> ATVAAYNLTWKSTNFKTILEWEPKPVNQVYTVQISTKSGDWKSKCFYTTDTECDLTDEIVKDVKQTYLARVFSYPAGNVESTGSAGEPLYENSPEF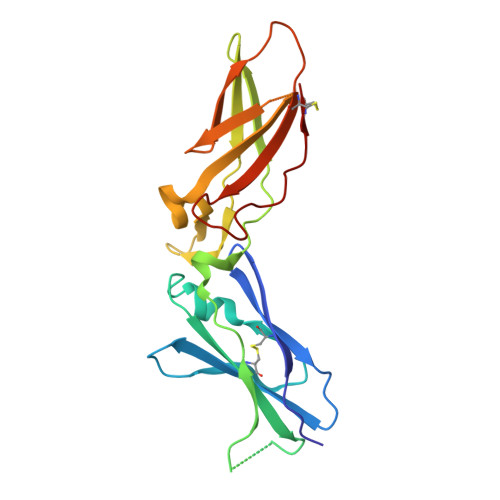TPYLETNLGQPTIQSFEQVGTKVNVTVEDERTLVRRNNTFLSLRDVFGKDLIYTLYYWKSSSSGKKTAKTNTNEFLIDVDKGENYCFSVQAVIPSRTVNRKSTDSPVECM2-[4-(ethylsulfonyl)phenyl]-N-[2'-fluoro-4'-(1,1,1,3,3,3-hexafluoro-2-hydroxypropan-2-yl)[1,1'-biphenyl]-4-yl]acetamide 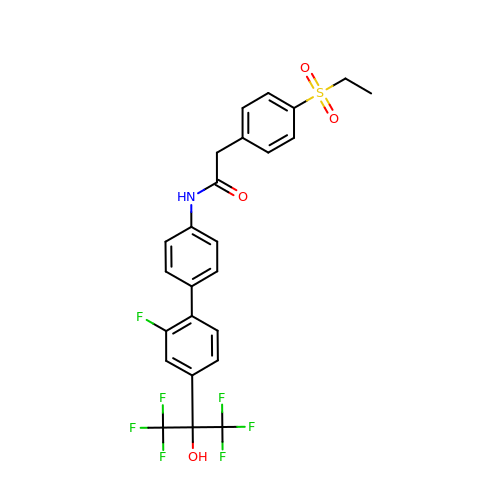| C25 H20 F7 N O4 S | AUIAOCHKUNGZHV-UHFFFAOYSA-N Human mitochondrial chaperonin mHsp60 is essential for mitochondrial function by assisting folding of mitochondrial proteins. Unlike the double-ring bacterial GroEL, mHsp60 exists as a heptameric ring that is unstable and dissociates to subunits. Due to its roles in human health, mHsp60 has been proposed as potential biomarkers and drug targets. mHsp60 belongs to an essential protein family called chaperonin that are conserved among the three kingdoms of life. The main function of chaperonins is to mediate folding of cellular proteins.

We purified active heptameric mHsp60, and determined a cryo-EM structure of mHsp60 heptamer at 3.4 Å. The map shows that the equatorial domain has the highest resolution (3.3 Å), while the apical domain has the lower resolution range (3.9–4.5 Å). The equatorial domains contribute most of the inter-subunit interactions, accounting for ~ 75% of the total inter-subunit interface and 44 residues involved in inter-subunit interactions. Center on the inter-subunit interface is a four-stranded β-sheet: β1 and β18 from one subunit connected with β2 and β3 from the other subunit. β strands are shorter in mHsp60 than in GroEL: 12 mHsp60 residues compared with 19 GroEL residues are involved in the β-sheet. Specifically, β1 and β18 are shortened to three residues, the minimal length for β-strands, from five and seven residues in GroEL, respectively. Thus, the three mHsp60 unique residues, T35, A516 and V112, diminish the restrains required to form the twisted conformations found in GroEL β2 and β18, leading to shortened β2 and β18 in mHsp60. Thus, the three mHsp60 residues, S57, D59 and E522, contribute to the shortened β1 and β18. Overall, mHsp60 has a much smaller inter-subunit interface than GroEL, ~ 1258 Å2 versus ~ 1674 Å2. Importantly, the unique sequences, T35, S57, D59, V112, A516, and E522, are specific to and conserved within the mitochondrial chaperonins of higher eukaryotes including human. Overall, the inter-subunit interface of the mHsp60 heptamer increases drastically by ~ 49% from 1258 Å2 in the mHsp60 alone structure to 1871 Å2 in the mHsp60-mHsp10 structure.

>[7x]AKDVKFGADARALMLQGVDLLADAVAVTMGPKGRTVIIEQSWGSPKVTKDGVTVAKSIDLKDKYKNIGAKLVQDVANNTNEEAGDGTTTATVLARSIAKEGFEKISKGANPVEIRRGVMLAVDAVIAELKKQSKPVTTPEEIAQVATISANGDKEIGNIISDAMKKVGRKGVITVKDGKTLNDELEIIEGMKFDRGYISPYFINTSKGQKCEFQDAYVLLSEKKISSIQSIVPALEIANAHRKPLVIIAEDVDGEALSTLVLNRLKVGLQVVAVKAPGFGDNRKNQLKDMAIATGGAVFGEEGLTLNLEDVQPHDLGKVGEVIVTKDDAMLLKGKGDKAQIEKRIQEIIEQLDVTTSEYEKEKLNERLAKLSDGVAVLKVGGTSDVEVNEKKDRVTDALNATRAAVEEGIVLGGGCALLRCIPALDSLTPANEDQKIGIEIIKRTLKIPAMTIAKNAGVEGSLIVEKIMQSSSEVGYDAMAGDFVNMVEKGIIDPTKVVRTALLDAAGVASLLTTAEVVVTEIP>[2x]GSTGSMFKLLLIFADPAEAARTLSLF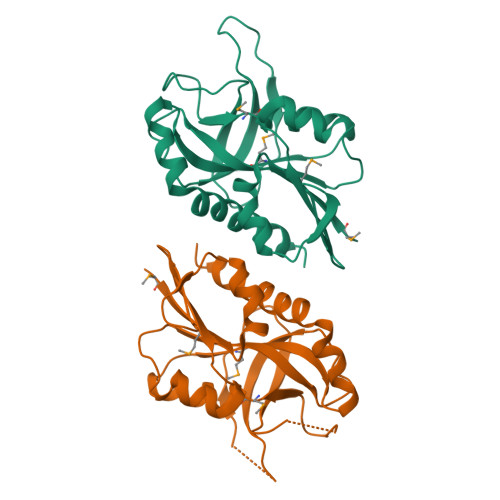PFSLNKENFYTYHTENVLLDVMVLKTWGYRGVVQALSPPPSGYDLWINAGFAGAANPNIPLLKTYTITSVKELTPTTSVEEELEVTPIPRLPLAQLTSVRSPYRDGFHEHLQLVDMEGFFIAKQASLVACPCSMIKVSSDYTTREGQDFLKNNKVKLSQKLAEAIFPIYSSFIDV> XXXXXXXXXXXSLKHLYSSIILIKNSRDESSSPYEWCIWQLKRCFAHQIETPQEVIPIIISVSSMDNKLSSRIIQTFCNLKYLKLDELTLKKVCGGILPLWKPELISGTREFFVKFMASIFMWSTRDGHDNNCTFSETCFYVLQMITNWVLDDKLIALGLTLLHDMQSLLTLDKIFNNATSNRFSTMAFISSLDILTQLSKQTKSDYAIQYLIVGPDIMNKVFSSDDPLLLSAACRYLVATKNKLMQYPSTNKFVRMQNQYIMDLTNYLYRNKVLSSKSLFGVSPDFFKQILENLYIPTADFKNAKFFTITGIPALSYICIIILRRLETAENTXXXXXXXXXXXXXXXXXXXXXXXXXXXXXXXXXXXVNNIHDLRVKILMHLSNTANPYRDIAAFLFTYLKSLSKYSVQNS;> MPYTWKFLGISKQLSLENGIAKLNQLLNLEVDLDIQTIRVPSDPDGGTAADEYIRYEMRLDISNLDEGTYSKFIFLGNSKMEVPMFLCYCGTDNRNEVVLQWLKAEYGVIMWPIKFEQKTMIKLADASIVHVTKENIEQITWFSSKLYFEPETQDKNLRQFSIEIPRESCEGLALGYGNTMHPYNDAIVPYIYNETGMAVERLPLTSVILAGHTKIMRESIVTSTRSLRNRVLAVVLQSIQFTSE;> MSNELRLEDNYVPTSDTLVVFKQLMKLPVTVLYDLTLSWFAKFGGSFDGDIYLLTETLDLLIEKGVRRNVIVNRILYVYWPDGLNVFQLAEIDCHLMISKPEKFKWLPSKALRGDGKPYVVKLQPAKFIENLQTDLAKIYHCHVYMFKHPSLPVLITRIQLFDSNNLFLSTPNIGSINKESLYNKLDKFQGKPLISRRPYYVAFPLNSPIIFHSVDKDIYARLVLQSISRTISERETIIFKPVQKIPVKSIHNIMTLLGPSRFAESMGPWECYASANFERSPLHDYKKHQGLTGKKVMVREFDDSFLNDDENFYGKEEPEIRRLRLEKNMIKFKGSANGVMDQKYNDLKEFNEHVHNIRNGKKNEDSGEPVYISRYSSLVPIEKVGFTLKNEINSRIITIKLKFNGNDIFGGLHELCDKNLINIDKVPGWLAGENGSFSGTIMNGDFQREQVAKGGLL;> MSRIDDLQQDIESLLSEINSLEESREKLKAKIKDKRKNEESANPIVQEFEDLFDQFPQLNNFLFNEHPELEETDDKDISRAQADIPATPIPYEPKKRAKLENEEILPEQEWVLKTQPMVQHQMFDPGVADLLDTDILTSPSKRKRKLKIDDISTSDRSELEDYIVLENVYRMFGITFFPLVDPIDLKIKDASGEIFVDREMLGIRLEVFSERTSQFEKPHYVLLKKRIKSNSWFLFKHTIPSFIDVQGIFDDTNGGLVISHDDAYLFAKRVFLQLVEVQKRRQIFKDLEAKKIIHDLDLDLESSMVSFFVKDIKVELFVKQNEIVSCSILDDIHDFSQNNKSKWEIALLGSLDDLELKLNHSFATIFK;> MDFTSDTTNSHDTSNSHLSLEDAVGTHHAGEADVNIDGDEKQQLSLLDDDQVRALKLQEEKDALLTRRNTLLQEIQTYQNILMKENNSKTKNGDILQNDITQDFLNLISISSSNPNSAISDRKRVERINGLTNLQKELVTKYDTLPLLNMNLRLSYLRDHTYPHLQVSVQSRDRVHNDGIEVLVVNYKFCRNTMNPFEIQFKMFYKFEDSTLLKWEILRISTNVRLKAKQLLATRNFQKCLLSLYEFDKIKSKKTGIFQNLINLLKRKTRCYLMNNSDSLIVERVIREGRLTTIKLQINFIITMPGERGKPRNCFLPMSKISIALWKGGERFNQIDLDEICYGLIKEYGVKTGLKEICNVCLFPDMYAR;> XXXXXXXXXXXXXXXSILRLLETNTVSALDSVFEKYEKEMNQMTHGDNNEVKRIYSKKERLLEIILTKIKKKLRQAKFPSRISERDLDIEYIYSKRQFIQNRYSQELQNNERLEAILSREQNLLEETRKLCMNLKTNNKKRLTEKLIQKDLHPVLNKAMEYTYGLESTNGFMHPDGPVTFRNDSHELNLMLNDPIKSTADVRLDKEEVLSLLPSLKEYTKKSKELKETMGQMISDSHEEEIKEVFVPHHESHQDKTEEDIH;> XXXXXXXXXXXXXXXXXXXXXXXXXXXFRKLLYKLDLRLFQTISDQMTRDLKDILDINVSNNELCYQLKQVLARKEDLNQQIISVRNEIQELKAGKDWHDLQNEQAKLNDKVKLNKRLNDLTSTLLGKYEGDRKIMSQDSEDDSIRDDSNILDIAHFVDLMDPYNGLLKKINKINENLSNELQPSL;> MTDTYNSISNFIENELTALLSSDDYLMDDLAGELPNEVCRLLKAQVIEKRKDAMSRGKQDLLSKEIYDNESELRASQSQQIMELVGDIPKYSLGSELRNRVEGEPQSTSIERLIEDVLKLPQMEVADEEEVEVENDLKVLSEYSNLRK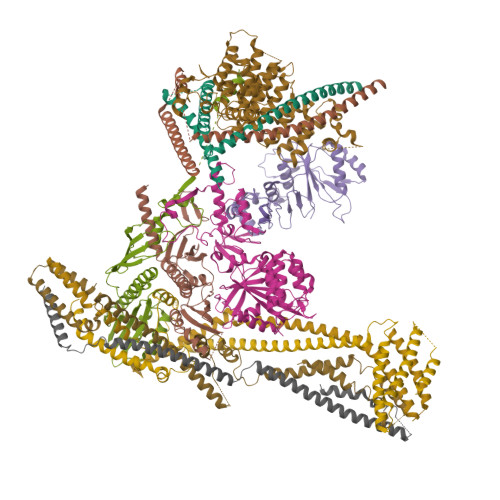DLILKCQALQIGESKLSDILSQTNSINSLTTSIKEASEDDDISEYFATYNGKLVVALEEMKLLLEEAVKTFGNSPEKREKIKKILSELKK;> MNSEQLLHNYVSDSLLTTLISFQEFKQQLQSYTSDEQQLQHWYELLQARDARVTSELEARIKQFFITLRSRLLRFLESEQLSHSLSLETLIDALYKINDLLQQRLQILDDAIQEKTSELAEFENMVRSPSAGDNAIPGLLQIIQSYINLLEEN> SSFQSTVDSDSADQKEYLISDTGGQQLSISDAFIKESLFNRRVEEKSKELPFTPLGWHHNNLELLREENGEKQAMERLLSANHNHMMALLQQLLHSDSLSSSWRDIIVSLVCQVVQTVRPDVKNQDDDMDIRQFVHIKKIPGGKKFDSVVVNGFVCTKNIAHKKMSSCIKNPKILLLKCSIEYLYREETKFTCIDPIVLQEREFLKNYVQRIVDVRPTLVLVEKTVSRIAQDMLLEHGITLVINVKSQVLERISRMTQGDLVMSMDQLLTKPHLGTCHKFYMQIFQLPNEQTKTLMFFEGCPQHLGCTIKLR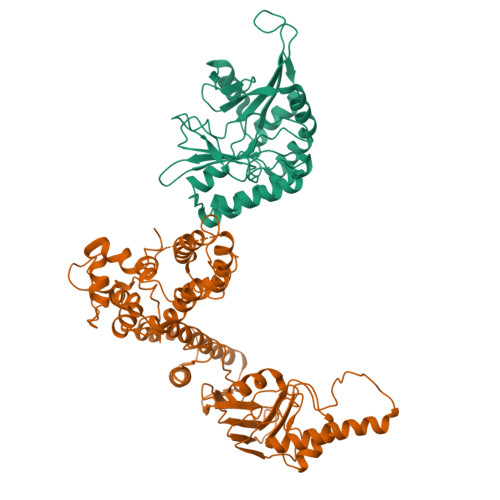GGSDYELARVKEILIFMICVAYHSQLEISFLMDEFAMPPTLMQNPSFHSLIEGRGHEGAVQEQYGGGSIPWDPDIPPESLPCDDSSLLELRIVFEKGEQENKNLPQAVASVKHQEHSTTACPAGLPCAFFAPVPESLLPLP;> CRLYYAGEFHKMREVILDSSEEDFIRSLSHSSPWQARGGKSGAAFYATEDDRFILKQMPRLEVQSFLDFAPHYFNYITNAVQQKRPTALAKILGVYRIGYKNSQNNTEKKLDLLVMENLFYGRKMAQVFDLKGSLRNRNVKTDTGKESCDVVLLDENLLKMVRDNPLYIRSHSKAVLRTSIHSDSHFLSSHLIIDYSLLVGRDDTSNELVVGIIDYIRTFTWDKKLEMVVKSTGILGGQGKMPTVVSPELYRTRFCEAMDKYFL>[2x]YVEFVAQISPQYPMFTVPLPIPPVKQPRLTVTNPVNGQEIWYYEVEIKPFTHQVYPDLGSADLVGYDGMSPGPTFQVPRGVETVVRFINNAEAPNSVHLHGSFSRAAFDGWAEDITEPGSFKDYYYPNRQSARTLWYHDHAMHITAENAYRGQAGLYMLTDPAEDALNLPSG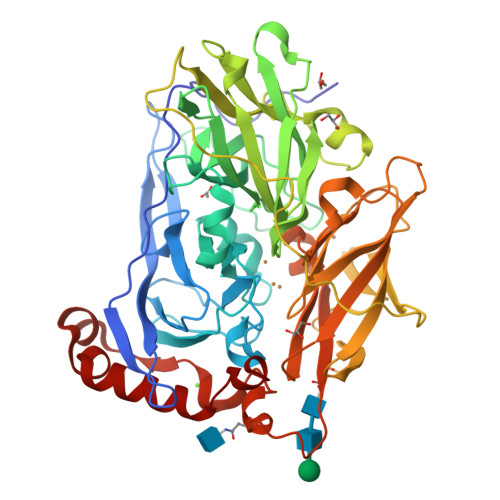YGEFDIPMILTSKQYTANGNLVTTNGELNSFWGDVIHVNGQPWPFKNVEPRKYRFRFLDAAVSRSFGLYFADTDAIDTRLPFKVIASDSGLLEHPADTSLLYISMAERYEVVFDFSDYAGKTIELRNLGGSIGGIGTDTDYDNTDKVMRFVVADDTTQPDTSVVPANLRDVPFPSPTTNTPRQFRFGRTGPTWTINGVAFADVQNRLLANVPVGTVERWELINAGNGWTHPIHIHLVDFKVISRTSGNNARTVMPYESGLKDVVWLGRRETVVVEAHYAPFPGVYMFHCHNLIHEDHDQMAAFNATVLPDYGYNATVFVDPMEELWQARPYELGEFQAQSGQFSVQAVTERIQTMAEYRPYAAADE>[2x]GPLGSMQYANAYQAYQHNRVSVESPAKLIEMLYEGILRFSSQAKRCIENEDIEKKIYYINRVTDIFTELLNILDYEKGGEVAVYLTGLYTHQIKV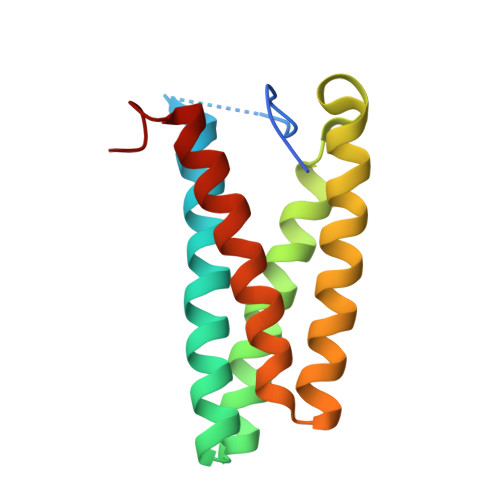LTQANVENDASKIDLVLNVARGLLEAWREIHSDELA>MGHHHHHHHHHLEKLASIDAQLRLLVPGKVSEDDKLIEYDALLLDKFLDILQDLHGEDLKEAVQECYELSAEYEGKHDPKKLEELGSVLTSLDPGDSIVIAKAFSHMLNLANLAEEVQIAYRRRIKLKRGDFADEANATTESDIEETFKKLVLKLNKSPEEVFDALKNQTVDLVLTAHPTQSVRRSLLQKHGRIRNCLAQLYAKDITPDDKQELDEALHREIQAAFRTDEIRRTPPTPQDEMRAGMSYFHETIWKGVPKFLRRVDTALKNIGINERVPYNAPLIQFSSWMGGDRDGNPRVTPEVTRDVCLLARMMASNMYFSQIEDLMFEMSMWRCNSELRVRAEELYRTARRDVKHYIEFWKQVPPTEPYRVILGDVRDKLYNTRERSRHLLAHGISDIPEEAVYTNVEQFLEPLELCYRSLCDCGDRVIADGSLLDFLRQVSTFGLSLVKLDIRQESDRHTDVLDAITQHLEIGSYREWSEEKRQEWLLAELSGKRPLFGSDLPKTEEVKDVLDTFNVLAELPSDCFGAYIISMATSPSDVLAVELLQRECHVKHPLRVVPLFEKLADLEAAPAAMARLFSIDWYRNRIDGKQEVMIGYSDSGKDAGRFSAAWQL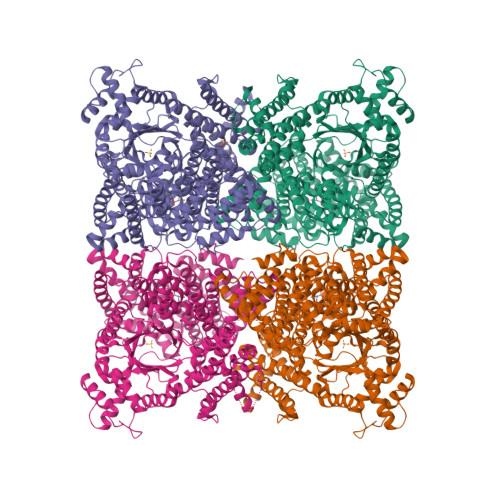YKAQEEIIKVAKEFGVKLVIFHGRGGTVGRGGGPTHLAILSQPPDTIHGSLRVTVQGEVIEQSFGEEHLCFRTLQRFCAATLEHGMNPPISPRPEWRELMDQMAVVATEEYRSIVFKEPRFVEYFRLATPELEYGRMNIGSRPSKRKPSGGIESLRAIPWIFAWTQTRFHLPVWLGFGAAFKHAIKKDSKNLQMLQEMYKTWPFFRVTIDLVEMVFAKGDPGIAALNDKLLVSEDLWPFGESLRANYEETKDYLLKIAGHRDLLEGDPYLKQRIRLRDSYITTLNVCQAYTLKRIRDPNYHVTLRPHISKEYAAEPSKPADELIHLNPTSEYAPGLEDTLILTMKGIAAGMQNTG[2x]> SEEAKPATTTTIKNTKPQCRPEDYATRLQDLRVTFHRVKPTLQREDDYSVWLDGTVVKGCWGCSVMDWLLRRYLEIVFPAGDHVYPGLKTELHSMRSTLESIYKDMR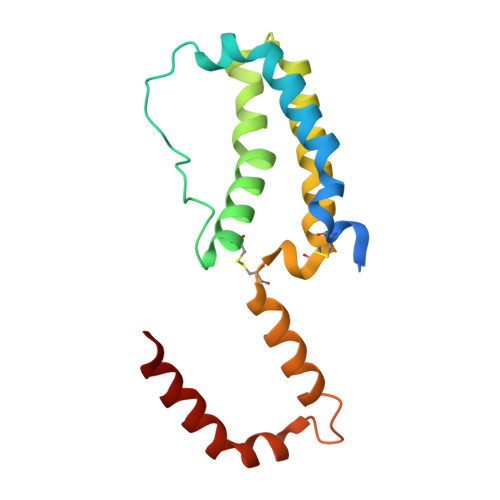QCPLLGCGDKSVISRLSQEAERKSDNGTRKGLSELDTLFSRLEEYLHSRK The ovarian tumor (OTU) family of deubiquitinases regulates diverse ubiquitin signals in humans. We have predicted and validated a set of OTU deubiquitinases encoded by several classes of pathogenic bacteria. By determining the ubiquitin‐bound structures of two examples, we demonstrate the novel strategies that have evolved to both thread an OTU fold and recognize a ubiquitin substrate. Our new bacterial OTU DUB structures allowed for the first cross‐kingdom structural analysis, from which we established a framework for identifying evolutionary adaptations in the S1 substrate‐binding site that impart DUB activity. This work establishes the OTU fold as a common tool used by bacteria to manipulate host Ub signaling and provides insight into the origins and adaptations of the OTU fold across eukaryotes, bacteria, and viruses.

The wMelOTU structure exhibits a pared‐down canonical OTU domain architecture with a central β‐sheet supported underneath by an α‐helical subdomain, but although additional α‐helical content typically sandwiches the β‐sheet from above, there is very little additional support in the wMelOTU structure (and EV3B). The core of the OTU fold that contains the active site (the central β‐sheet and two most proximal supporting α‐helices) closely resembles other OTU domains such as OTUB1 (1.6 Å RMSD) and vOTU (Fig EV3B, 1 Å RMSD), whereas the surrounding areas of structure are more divergent (Akutsu et al, 2011; Juang et al, 2012). Two regions of structure near the S1 substrate recognition site, encompassing 6 and 7 amino acids, respectively, are missing from the electron density (Figs 3A and EV3A). The structure confirms our prediction and mutagenesis of active site residues. However, the catalytic triad is misaligned as a result of the loop preceding the general base His (the so‐called His‐loop) occupying a descended conformation that would also occlude entry of the Ub C‐terminus into the active site. Thus, while the apo wMelOTU structure validates our prediction of an OTU fold, it raised new questions as to the mechanisms of substrate recognition. Our structure of wMelOTU shows that its sequence topology matches the most typical OTU arrangement seen in OTUB1 and vOTU, and we would predict BurkOTU, RickOTU, and wPipOTU to be similar as well.

> MTTAKKRKLPSDLHDVEVGIKRPRISGQEITLLNSNPYPDNFYVGQAIGNGSCFFDSFRQSLEQQTGEQVTAEKLRNDCREFAQKNPPKWFTNAIVNSHDNNGQHRSETVDNYTADIMRNSRWGDPDVEGRILCEKYKVKLHVIENQTVDNQDLSLHELIDNSGSKSAGEYNKVDYDDSSTVHIINKGGLHFEPLLDRNKSSAKQLQEQEDFLLA> MPFEIVFEGAKEFAQLIDTASKLIDEAAFKVTEDGISMRAM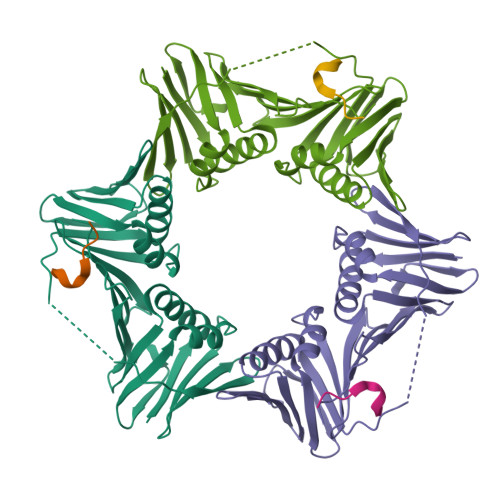DPSRVVLIDLNLPSSIFSKYEVVEPETIGVNLDHLKKILKRGKAKDTLILKKGEENFLEITIQGTATRTFRVPLIDVEEMEVDLPELPFTAKVVVLGEVLKDAVKDASLVSDSIKFIARENEFIMKAEGETQEVEIKLTLEDEGLLDIEVQEETKSAYGVSYLSDMVKGLGKADEVTIKFGNEMPMQMEYYIRDEGRLTFLLAPRVEE;> XKQATLFDFLKK(2S)-2-[(1R,3aS,4E,7aR)-7a-methyl-4-[2-[(3R,5R)-4-methylidene-3,5-bis(oxidanyl)cyclohexylidene]ethylidene]-2,3,3a,5,6,7-hexahydro-1H-inden-1-yl]oct-4,6-diene-3-one 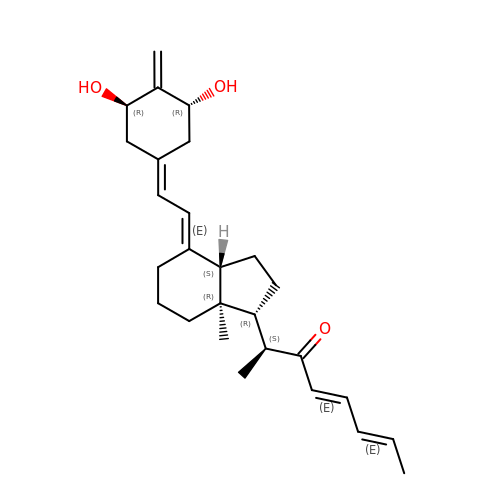| C27 H38 O3 | NXEUFUPQFMVYDT-SVJWBRFGSA-N> TVIKNETGTISISQLNKNVWVHTELGSFNGEAVPSNGLVLNTSKGLVLVDSSWDDKLTKELIEMVEKKFQKRVTDVIITHAHADRIGGIKTLKERGIKAHSTALTAELAKKNGYEEPLGDLQTVTNLKFGNMKVETFYPGKGHTEDNIVVWLPQYNILVGGCLVKSTSAKDLGNVADAYVNEW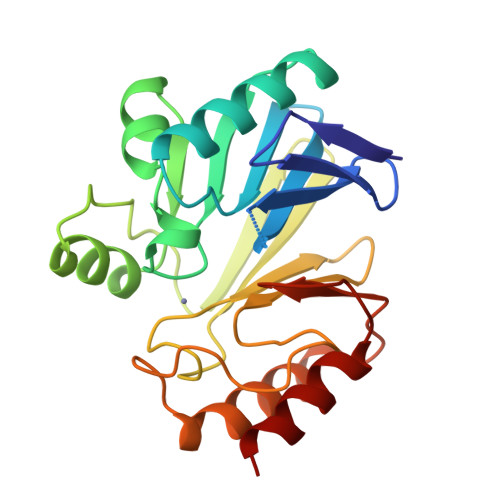STSIENVLKRYRNINAVVPGHGEVGDKGLLLHTLDLLK>[3x]MSNPSLVIVSPALPGANNGNWRTAQRWKALLSPVCSARVVQQWPDADASADTVMLALHARRSAESIAHWAHAHPGRGLGVVLTGTDLYQDIGSDPQAQRSLQLAQRLVVLQALGAEALPPECRAKARVVYQSTSARAELPKSARQLRAVMVGHLRQVKSPQTLFDAARLLCGREDIRIDHIGDAGDAGLGELARALASDCPGYRWLGALPHAQTRQRIQRAHVLVHTSALEGGAHVIMEAVRSGTPVLASRVPGNVGMLGNDYAGYFPHGDAAALAALLEACRAGQGSKDRAAGLLDSLRTQCALRAPLFDPRAEQAALFQLLNELQPPPP

A specific SEN biosynthetic pathway was identified in Variovorax paradoxus DSM 30034, which is recognized as a way to incorporate Se into organic matter in bacteria. The bacterial SEN biosynthesis gene cluster encodes three proteins, SenA, SenB, and SenC. SenB catalyzes the generation of the key intermediate selenoglucose product using SeP synthesized by selenophosphate synthetase (named SelD or SenC)15. In contrast to other types of GTs, SenB performs dual functions in two-step catalytic reactions, catalyzing the formation of C–Se glycosidic bonds and the subsequent cleavage of Se-P bonds to generate the final product.

To elucidate the structural basis leading to substrate recognition and the catalytic mechanism of SenB, we solved the structures of SenB complexed with various sugar donors, including the ternary complex SenB/UDP-Glc/PO43- (1.95 Å) and two binary complexes, SenB/UDP-GlcNAc (1.88 Å) and SenB/UDP-GalNAc (1.64 Å). In all solved crystal structures, each asymmetric unit contains three copies of SenB, which are unlikely to be functionally related due to the lack of protein‒protein interactions between them. Structural superposition of SenB/UDP-Glc, SenB/UDP-GlcNAc and SenB/UDP-GalNAc indicated that the spatial positions of the UDP moieties of the three sugar donors overlapped well. In our solved complex structures of SenB, the electron densities of the three different sugar moieties of the UDP-sugars were well defined. UDP-GlcNAc and UDP-GalNAc are a class of sugar donors with large spatial dimensions due to the presence of an N-acetyl group on the C-2′ of the sugar moiety. The acetyl groups in UDP-GlcNAc and UDP-GalNAc may enhance the affinity of SenB for additional hydrophobic interactions with V157 compared to that of other UDP-sugars. Weakening this interaction by altering V157 to various amino acids (A/F/I/M/R/K) decreased the activity of all mutants, yet these enzymes retained some catalytic function. The preference of SenB is as follows: UDP-GlcNAc > UDP-GalNAc > UDP-Glc > UDP-Gal > UDP-Rha > UDP-Xyl. Given the chemical structure and catalytic activity of the sugar donor, these findings suggest that the N-acetyl group of C-2′ and the hydroxymethyl group of C-5′ on the sugar moiety contribute to the catalytic efficiency of SenB. Using UDP-GlcNAc and UDP-GalNAc as sugar donors, the corresponding selenophosphate sugar intermediates catalyzed by the K158A mutant were detected through LC‒MS.Surface layers (S-layers) are proteinaceous crystalline coats that constitute the outermost component of most prokaryotic cell envelopes. In cells of the bacterial species Caulobacter crescentus (also known as Caulobacter vibrioides), the S-layer is composed of a single 1,026-amino acid residue SLP called RsaA (Smit et al., 1992). RsaA has a canonical bipartite arrangement, with a lattice-forming C-terminal domain (RsaACTD), consisting of residues 251–1,026, and a cell-anchoring N-terminal domain (RsaANTD), consisting of residues 1–250. The assembly of the RsaA S-layer is divalent metal-ion dependent (Nomellini et al., 1997; Bharat et al., 2017; Herrmann et al., 2020), as, without divalent metal ions, S-layer formation is inhibited both in vitro and on cells (Bharat et al., 2017).

Furthermore, cryoelectron microscopy (cryo-EM) and cryoelectron tomography (cryo-ET) investigations have demonstrated that binding of RsaA to lipopolysaccharide (LPS) molecules on the C. crescentus cell surface is also regulated by Ca2+ ions (von Kügelgen et al., 2020). Based on previous structural biology data, full-length RsaA has been predicted to contain 22 putative Ca2+-binding sites; 19 in RsaACTD (Bharat et al., 2017) (numbered 1–19) and three in RsaANTD (numbered 20–22) (von Kügelgen et al., 2020). To verify the Ca2+-binding sites in RsaANTD, we reconstituted the RsaANTD:PS (RsaA bound to the O-antigen oligosaccharide of LPS) complex (von Kügelgen et al., 2020) in vitro, in the presence of Ho3+ ions. Ho3+ has a high propensity to replace Ca2+ ions (Weis et al., 1991) and we wanted to use this property to spatially confirm the location of Ca2+ ions in each RsaANTD monomer. We performed cryo-EM single-particle analysis of the reconstituted complex, producing a 4.3-Å resolution map. Comparing this Ho3+-bound cryo-EM structure with a Ca2+-bound structure solved previously (von Kügelgen et al., 2020) showed strong densities in the region of one of the proposed Ca2+-binding sites. The proximity between this Ca2+ ion and the previously resolved LPS-binding pocket suggests that it might play a role in stabilizing the RsaANTD:PS complex, in line with previous results (von Kügelgen et al., 2020). (A) Density map of RsaANTD:PS complex supplemented with 5 mM Ho3+ before vitrification shown as black mesh at a contour level of 20 σ. Site 21 in RsaANTD could be replaced with Ho3+ and observed with single-particle cryo-EM, suggesting strongly that it is a Ca2+-binding site. Since all three proposed Ca2+ ion sites (sites 20–22) in RsaANTD were stable in MD simulations, we expect that these are probably also true Ca2+-binding sites, with sites 20 and 22 having less propensity to be replaced by Ho3+ under the conditions used, or Ho3+ is not capable of substituting for Ca2+ in these sites.

> AYTTAQLVTAYTNANLGKAPDAATTLTLDAYATQTQTGGLSDAAALTNTLKLVNSTTAVAIQTYQFFTGVAPSAAGLDFLVDSTTNTNDLNDAYYSKFAQENRFINFSINLATGAGAGATAFAAAYTGVSYAQTVATAYDKIIGNAVATAAGVDVAAAVAFLSRQANIDYLTAFVRANTPFTAAADIDLAVKAALIGTILNAATVSGIGGYATATAAMINDLSDGALSTDNAAGVNLFTAYPSSGVSGSENLYFQ> KHKILHRLLQ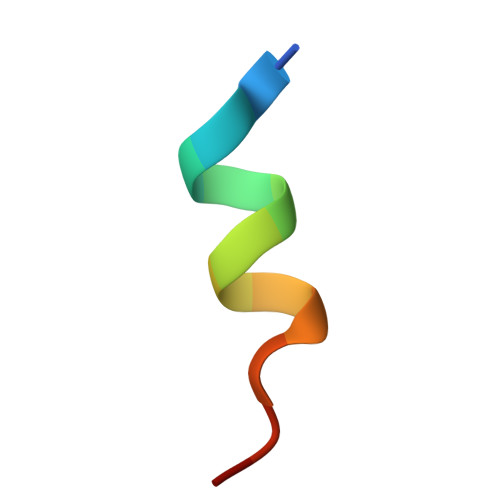DSSY> MKELIYIHEPNILFANGQKCADPRDGLALFGPFTKIYGIKSGVVGTQYGLSIFKNYINHIQKPIYNANNITRPMFPGFEAVFGCKWDADNVVFKEVTKEEIEKILYTESNHKRTYDLVSLFINKIITANKNEDEKVDVWFLVIPDEIYQYCRPNSVLPKDLVQTKSLITKSKAKSFRYEPTLFENINKELKEQEKEAITYNYDAQFHDQLKARLLEHTIPTQILRESTLAWRDFKNKFGAPKRDFSKIEGHLAWTISTAAFYKAGGKPWKLSDIRSGVCYLGLVYKQIEKSSNPKNACCAAQ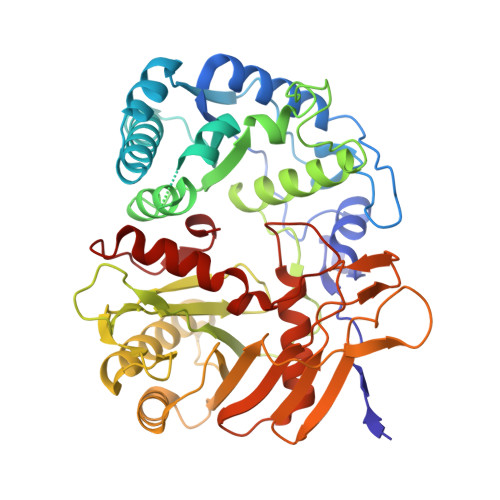MFLDNGDGTVFKGEVGPWYNQEKHEFHLNPKEAKALLTQALNSYKEQNGVFPKEIFIHAKTKFNGQEWNAFQEVTPEGTNLVGVTITKTKPLKLFKSEGNYPIMRGNAFIVNERSAFLWTVGYVPKTESTLSMEVPNPIFIEINKGEADIEQVLKDVLALTKLNYNACIYADGVPVTLRFADKIGEILTASTELKAPPLAFKYYI>[3x]AAFSGPKIAFYVGLKSPHEGYEVLKFDDVVTNLGNHYDPTTGKFSCQVRGIYFFTYHILMRGGD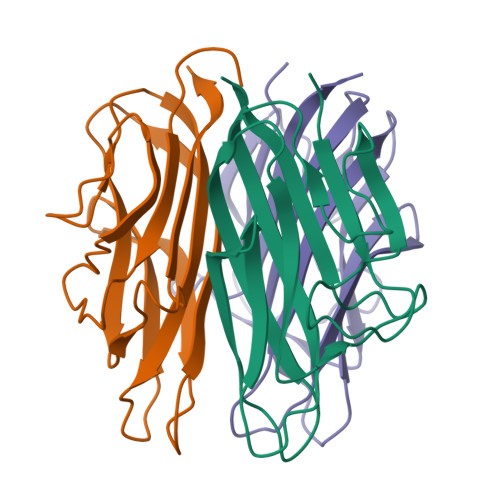GTSMWADLCKNGQVRASAIAQDADQNYDYASNSVVLHLDSGDEVYVKLDGGKAHGGNNNKYSTFSGFLLYPD> ACGGACACGTCA;> CACAC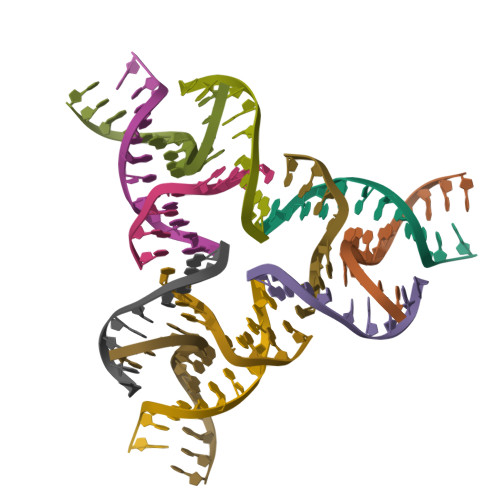CGT;> CTGACGTGTGCTC;> GGAGCTGTG> MVNAIRTPDQRFSNLDQYPF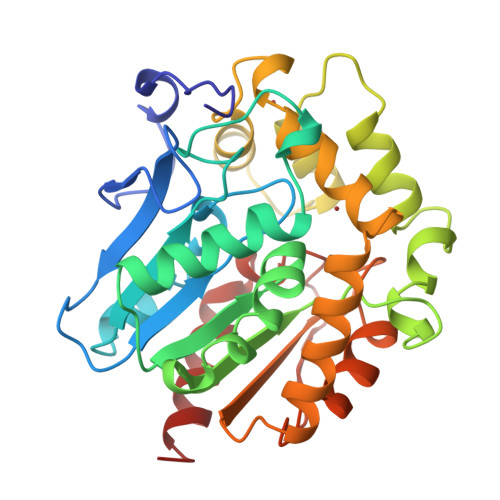SPNYLDDLPGYPGLRAHYLDEGNSDAEDVFLCLHGEPTWSYLYRKMIPVFAESGARVIAPDFFGFGKSDKPVDEEDYTFEFHRNFLLALIERLDLRNITLVVQDWGGFLGLTLPMADPSRFKRLIIMNACLMTDPVTQPAFSAFVTQPADGFTAWKYDLVTPSDLRLDQFMKRWAPTLTEAEASAYAAPFPDTSYQAGVRKFPKMVAQRDQACIDISTEAISFWQNDWNGQTFMAIGMKDKLLGPDVMYPMKALINGCPEPLEIADAGHFVQEFGEQVAREALKHFAETE>[2x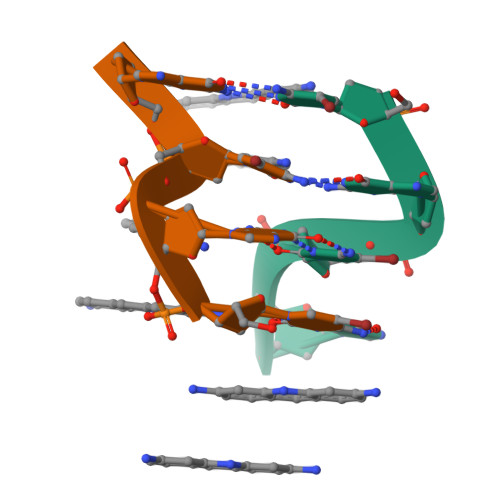]CGCG> HHHHHHHMDITKVDTSGASEITARQDKLTLQGVDAS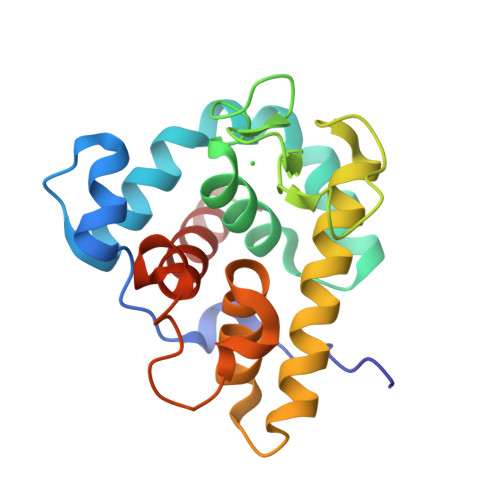HKLAEHDLVRMNKYKELITRVGQKHGLDPAIIAGIISRESRAGSALDHGWGDHGKGFGLMQVDKRYHKIVGAWDSEKHISQGTEILIEFIRRIQAKFPVWPKEHQLKGGISAYNAGDKNVRTYERMDVGTTGGDYSNDVVARSQWFKSQGY;> AGKNVNVEFRKGHSSAQYSGEIKGYDYDTYTFYAKKGQKVHVSISNEGADTYLFGPGIDDSVDLSRYSPELDSHGQYSLPASGKYELRVLQTRNDARKNKTKKYNVDIQIK>MKKSYLLAALIFFLAGLLHGTAFAMSGKSSKALNEAAEQGDLAKVKNLVQKNKIDLNAQDETGMTPLMNAAMGGNLDIVKFLLSKKVNLELKNNGGETALAFAVTNDAYDVAEELIKAGANVDIIVAGDEGDTLFMRAAQNNKKTAESILAKNKSLINKANTLGETALFAVARYGTPADIDFLIKKGADLKLKNKKGQTALDVAKEASNQDTAKALSKKKLEHHHH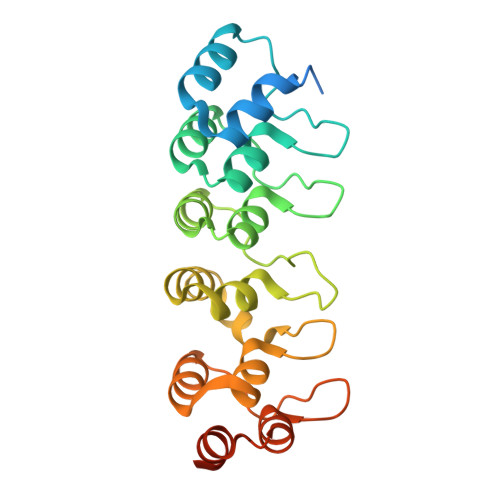HHHH[5x]>[4x]MKKIEILIVVDCAGA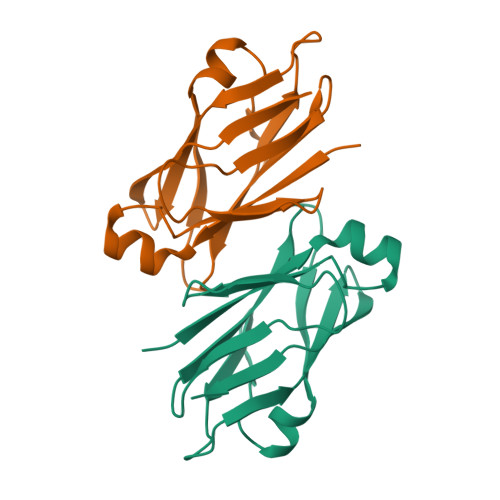LATTSLISNVYLIDSNQWLGSWDEGTCQLHTVSEDGQFICWRSCAISPDDEVNITGFYGDMIDQKACLPSPVNDAWEGRVQTRGDTGRYLYTISLSINGITMNFSPYLEVQ> SEGEADLYLDQYNFTTTAAIVSSVDRKIFVLLRDGRMLFGVLRTFDQYANLILQDCVERIYFSEENKYAEEDRGIFMIRGENVVMLGEVDIDKEDQPLEAMERIPFKEAWLTKQKNDEKRFKEETHKGKKMARHGIVYDFHKSDMY;> SENLYFQGSGSLFFSFFKTLVDQEVVVELKNDIEIKGTLQSVDQFLNLKLDNISCTDEKKYPHLGSVRNIFIRGSTVRYVYLNKNMVDTNLLQDATRREVMTERK;> METPLDLLKLNLDERVYIKLRGARTLVGTLQAFDSHCNIVLSDAVETIYQLNNEELSESERRCEMVFIRGDTVTLISTPSEDDDGAVEI;> MLPLYLLTNAKGQQMQIELKNGEIIQGILTNVDNWMNLTLSNVTEYSEESAINSEDNAESSKAVKLNEIYIRGTFIKFIKLQDNIIDKVKQQINSNNNSNSNGPGHKRYYNNRD;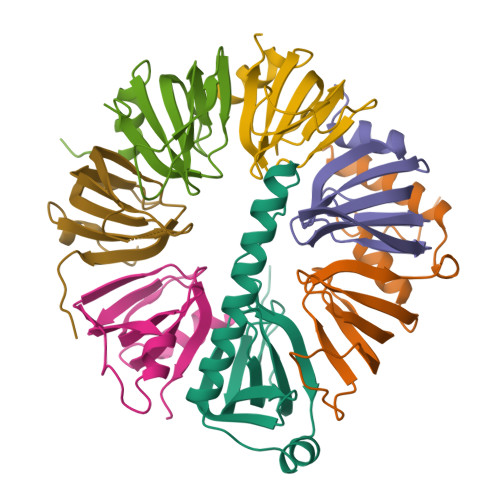> MSLPEILPLEVIDKTINQKVLIVLQSNREFEGTLVGFDDFVNVILEDAVEWLIDPEDESRNEKVMQHHGRMLLSGNNIAILVPGGKKTPTEAL;> MSGKASTEGSVTTEFLSDIIGKTVNVKLASGLLYSGRLESIDGFMNVALSSATEHYESNNNKLLNKFNSDVFLRGTQVMYISEQKI;> MHQQHSKSENKPQQQRKKFEGPKREAILDLAKYKDSKIRVKLMGGKLVIGVLKGYDQLMNLVLDDTVEYMSNPDDENNTELISKNARKLGLTVIRGTILVSLSSAEGSDVLYMQK>MNFEGKIALVTGASRGIGRAIAETLAARGAKVIGTATSENGAQAISDYLGANGKGLMLNVTDPASIESVLEKIRAEFGEVDILVNNAGITRDNLLMRMKDEEWNDIIETNLSSVFRLSKAVMRAMMKKRHGRIITIGSVVGTMGNGGQANYAAAKAGLIGFSKSLAREVASRGITVNVVAPGFIETDMTRALSDD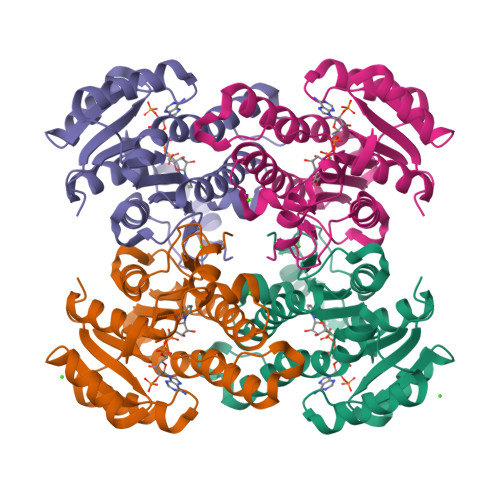QRAGILAQVPAGRLGGAQEIANAVAFLASDEAAYITGETLHVNGGMYMV[4x]> DENASAAEQVNKTIIGIDPGSGIMSLTDKAMKDYDLNDWTLISASSAAMTATLKKSYDRKKPIIITGWTPHWMFSRYKLKYLDDPKQSYGSAEEIHTITRKGFSKEQPNAAKLLSQFKWTQDEMGEIMIKVEEGEKPAKVAAEYVNKHKDQIAEWTK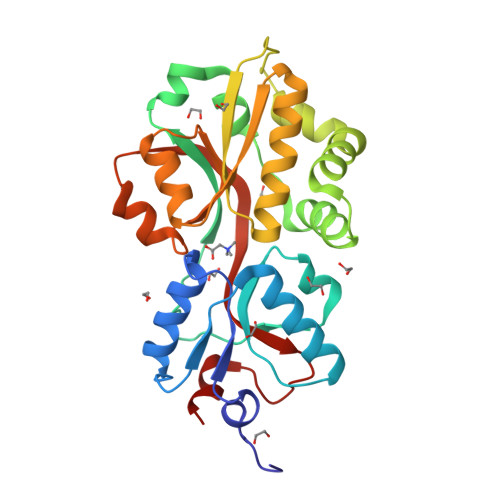GVQKVKGDKINLAYVAWDSEIASTNVIGKVLEDLGYEVTLTQVEAGPMWTAIATGSADASLSAWLPNTHKAYAAKYKGKYDDIGTSMTGVKMGLVVPQYMKNVNSIEDLKK The second and third steps of the histidine biosynthetic pathway (HBP) in plants are catalyzed by a bifunctional enzyme–HISN2. The enzyme consists of two distinct domains, active respectively as a phosphoribosyl-AMP cyclohydrolase (PRA-CH) and phosphoribosyl-ATP pyrophosphatase (PRA-PH). In this work, we obtained crystal structures of HISN2 enzyme from Medicago truncatula (MtHISN2) and described its architecture and interactions with AMP. The enzyme dimer is formed by two mutually swapped polypeptide chains, forming a bilobial protein—each domain forms one lobe.

MtHISN2-AMP complex crystallized in the C2 space group but with different unit cell parameters and six protein chains (three dimers) in the ASU. In the MtHISN2-AMP complex, AMP molecules were found near MBSs in both domains, PRA-PH and PRA-CH. AMP bound in the PRA-PH domain formed hydrogen bonds through the phosphate moiety and the adenine ring. The adenine N1 atom interacted with the Arg263 guanidine group. We also observed the π-π stacking between the adenine ring and the Tyr240 side chain; the approximate inter-ring distance was 3.6 Å. The proposed orientation of the adenine ring of PR-ATP was rotated by ~ 180° in the ring’s plane to the AMP pose in the MtHISN2-AMP complex. This means that the binding of AMP to the PRA-PH domain in our MtHISN2 complex apparently shows the positioning of the N1-phosphoribosyl of PR-ATP and the plane of its adenine ring. The second AMP binding site was located within the PRA-CH domain. The phosphate moiety formed an extensive network of hydrogen bonds with surrounding residues. We also observed edge-to-face interaction between the aromatic rings of the adenine and Trp107, with ≈ 3.5 Å distance and angle ω ≈ 45°. However, we did not observe a metal cation bound at MBS4 in the MtHISN2-AMP complex, suggesting that a metal bound to the MBS4 can either promote substrate binding or may not be physiologically relevant. Distances observed in the MtHISN2-AMP complex, Zn2+…H2O of 2.4 Å, Nδ of His143…H2O of 3.0, and H2O…C6 of 3.1 Å, are consistent with this mechanism.

>SNAVDSLLDSVKWDNKGLAVAIAQNVDTGAILMQGFANREAVATTISSRKATFYSRSRSSLWTKGETSNNFINVHDVFLDCDRDSIIYLGKPDGPTCHTGAETCYYTPVFDLLKEEEVEGNKLALTSLYALESTISQRKAEVVEENGKPSWTKRLLLNDKLLCSKIREEANELCETLENNEDKSRTASEMADVLYHAMVLLALKDVKVEEVLQVLRQRFSKSGIEEKRSRPTQKSVEN[6x]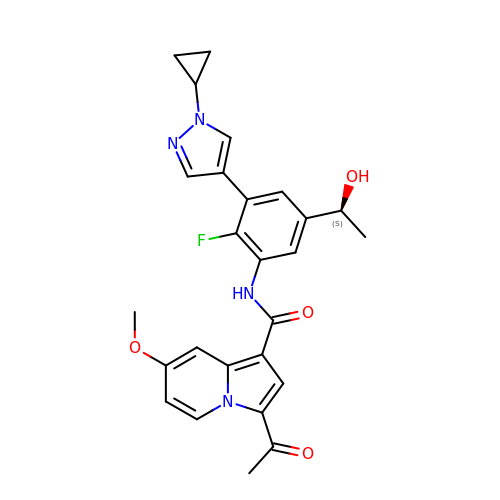N-[3-(1-cyclopropylpyrazol-4-yl)-2-fluoranyl-5-[(1S)-1-oxidanylethyl]phenyl]-3-ethanoyl-7-methoxy-indolizine-1-carboxamide | C26 H25 F N4 O4 | KKCORLIQMAQULG-AWEZNQCLSA-N>[2x]AMAGVFTYETEFTSVIPPPRLFKAFILDADNLIPKIAPQAVKCAEIIEGDGGVGTIKKITFGEGSQFGSVTHKIDGIDKENFVYSYSLIEGDALSDKIEKISYETKLVSSSDGGSIIKSTSNYHTKGDVEIKEEHVKAGKEKFSHLFKLVEGYLLANPNEYC

Here, a series of new methods are presented based on the use of a low X-ray-background film as a crystallization support and a photoablation laser that enable the automation of major operations required for the preparation of crystals for X-ray diffraction experiments. In this approach, the controlled removal of the mother liquor before crystal mounting simplifies the cryocooling process, in many cases eliminating the use of cryoprotectant agents, while crystal-soaking experiments are performed through diffusion, precluding the need for repeated sample-recovery and transfer operations. We have previously shown that the transfer of crystals to X-ray data-collection pins can be automated through the so-called CrystalDirect approach, which relies on the use of a thin, low X-ray-background film as a crystallization support from which crystals are recovered by excising the film with a laser beam and attaching it to an X-ray data-collection pin. The CrystalDirect system enables the automation of sample mounting and cryocooling and can contribute to closing the automation gap that currently exists between crystallization and X-ray data collection.

Some of these crystals grew in conditions that require the addition of cryoprotectants when processed by standard manual methods. However, in all cases tested the automated laser mounting and direct cryocooling after liquid removal with the CrystalDirect robot produced samples with very good diffraction properties leading to high-quality structural models.> REQVKDSNGNPVKRGAKYFIQPAKSNGGGLVPAAINILPFCPLGITQTLLPYQPGLPVSFGYEPVIVGTDYIYTSTTINIEFRSEIWPVCNELSKLWAVDVSSSAAKEPAIIIGGERTAPNSLFKIEEATGAHTYKLTTSSGTVGTIPGPWLGAPQLIATNDDAKTLFVKFVKVDDDAT

WSCPs are a class of non-photosynthetic Chl-binding proteins from plants. These homo-tetrameric proteins are present only in the plant family of Brassicaceae and contain only one Chl per monomer in symmetrically related and structurally identical binding sites. Interestingly, different WSCPs are characterized by different relative affinities for Chl a or Chl b. To this end, we coupled a crystallographic approach, solving the still missing Chl b-reconstituted wt structures (Chl b Lv-wt and Chl b Bo-wt), to a Raman investigation focused on the carbonyl groups, with the aim to characterize the (possible) H-bond in which the carbonyl may be involved.

The 2 amino acids-longer motif (-PVCNEL-) found in Bo-wt at the corresponding position does not lead to a preference for either Chl a or Chl b. The increased length of the PVCNEL motif forces the potential H-bond partner (backbone nitrogen of V89) away from the C-71 carbonyl, resulting in a distance between the backbone nitrogen of V89 and the formyl oxygen of pyrrole ring B of 4.0 Å. In Bo-wt, the increased distance of the first suitable H-bond donor in the backbone of the PVCNEL motif seems to be compensated by an alternative H-bond donor at a suitable distance from the formyl group. Its assignment to a water molecule is based on the small available space inside the binding pocket and to the faintness of its electron density in the crystallographic structure. Therefore, the position of the water molecule inside the Chl binding pocket appears to be not rigidly defined, both in the crystal and in solution. Bo-wt also has a proline residue in the binding pocket, close to ring B, but the residue conformation is not affected by the binding of Chl b and a water molecule, as it retains its endo-conformation. Additionally, the Raman characterization proved to be fundamental also in the case also of Bo-wt, as it allowed to reveal the presence of an H-bond partner for the bound Chl b, not discernible in the crystallographic structure due to the flexibility of the binding site. Accordingly, when the surrounding of ring B is less hindered, like in Bo-wt, there is little or no selectivity.> SLN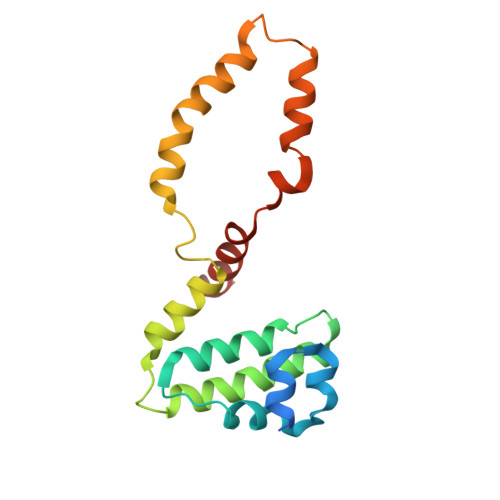TGEPAPVLSSPPPADVSTFLAFPSPEKLLRLGPKSSVLIAQQTDTSDPEKVVSAFLKVSSVFKDEATVRMAVQDAVDALMQKAFNSSSFNSNTFLTRLLVHMGLLKSEDKVKAIANLYGPLMALNHMVQQDYFPKALAPLLLAFVTKPNSALESSSFARHSLLQTLYKV>[2x]GVSETAPASRRGELAVCDAVSGWVTDRRTAVDLRGREVEVLGEVPAAGGSPLRQYFFETRCKADNAEEGGPGAGGGGCRGVDRRHWVSECKAKQSYVRALTADAQG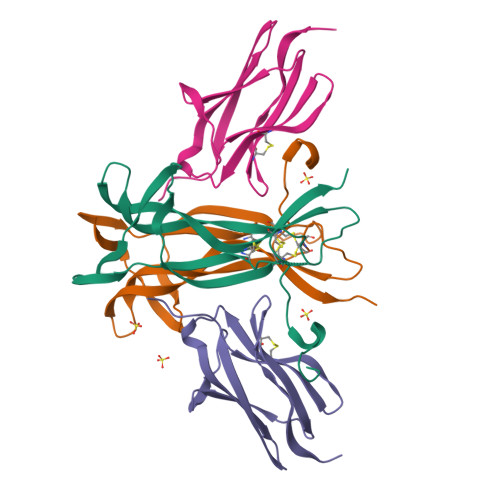RVGWRWIRIDTACVCTLLSRTGRA;>SHMAPTITFLESPTSDHHWCIPFTVKGNPKPALQWFYNGAILNESKYICTKIHVTNHTEYHGCLQLDNPTHMNNGDYTLIAKNEYGKDEKQISAHFMGWPG[2x]>[4x]MSKPDDPAYHWNGAELDLDAYLARIGFAGERAPTLATLRELVYRHTTAIPFENLEAVLGRPVRLDLATLQDKLVHSRRGGYCYENAGLFAAALERLGFGVTGHTGRVTMGAGGLRPATHALLRVTTADDDRVWMCDVGFGRGPLRPYELRPQPDEFTLGDWRFRLERRTGELGTDLWVLHQFGRDGWVDRYTFTTAPQYRIDFEVGNHFVSTSPRSPFTTRPFLQRFHSDRHHVL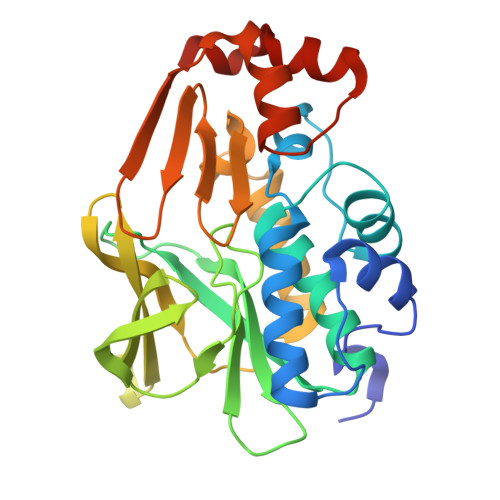DGLTLITERPDGSADIRALTPGELPEVINELFDIELPGPDLDALTTGSWLERVAAGTP> SNAIQDNGATTAAQTVAMPTIDES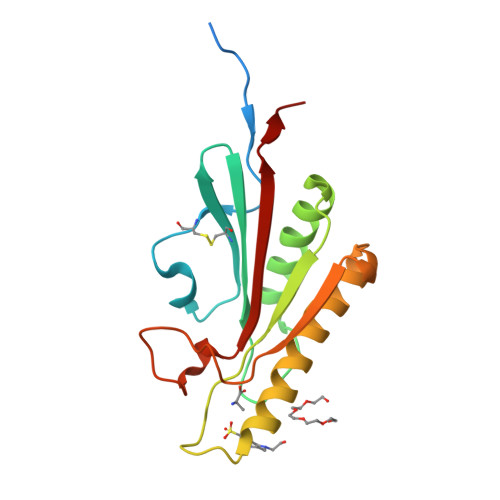KYVLPAGIKQCEGNFNLTEDGVACYTINGDDVTVYLDTKFAYDKATLNAKGKKAIASFVNFIKDSNISSVTVKGYASQGQTGSEFDIYNQKLSEKRAQAVADYMKQLGLDSEKIITKGFGYNDTLGGIHKSDPRNQRVEASVSAPLKEAN> KDRISWLGQPMKIEENRTYYQKVSIDEEMLEVGDCVSVIPDDSSKPLYLARVTALWEDKNGQMMFHAHWFCAGTDTVLGATSDPLELFLVGECENMQLSYIHSKVKVIYKAPSENWAMEGGTDPETTLPGAEDGKTYFFQLWYNQEYARFESPPKTQPTEDNKHKFCLSCIRLAELRQKEMPKVLEQIEEVDGRVYCSSITKNGVVYRLGDSVYLPPEAFTFNIKVASPVKRPKKDPVNETLYPEHYRKYSDYIKGSNLDAPEPYRIGRIKEIHCGKKKGKVNEADIKLRLYKFYRPENTHRSYNGSYHTDINMLYWSDEEAVVNFSDVQGRCTVEYGEDLLESIQDYSQGGPDRFYFLEAY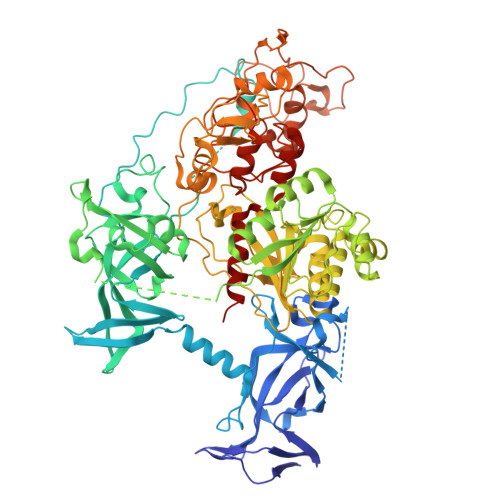NSKTKNFEDPPNHARSPGNKGKGKGKGKGKGKHQVSEPKEPEAAIKLPKLRTLDVFSGCGGLSEGFHQAGISETLWAIEMWDPAAQAFRLNNPGTTVFTEDCNVLLKLVMAGEVTNSLGQRLPQKGDVEMLCGGPPCQGFSGMNRFNSRTYSKFKNSLVVSFLSYCDYYRPRFFLLENVRNFVSYRDSMVLKLTLRCLVRMGYQCTFGVLQAGQYGVAQTRRRAIILAAAPGEKLPLFPEPLHVFAPRACQLSVVVDDKKFVSNITRLSSGPFRTITVRDTMSDLPEIQNGASNSEIPYNGEPLSWFQRQLRGSHYQPILRDHICKDMSPLVAARMRHIPLFPGSDWRDLPNIQVRLGDGVIAHKLQYTFHDVKNGYSSTGALRGVCSCAEGKACDPESRQFSTLIPWCLPHTGNRHNHWAGLYGRLEWDGFFSTTVTNPEPMGKQGRVLHPEQHRVVSVRECARSQGFPDSYRFFGNILDRHRQVGNAVPPPLAKAIGLEIKLCLLSSA> MRVLVTGGSGYIGSHTCVQLLQNGHDVIILDNLCNSKRSVLPVIERLGGKHPTFVEGDIRNEALMTEILHDHAIDTVIHFAGLKAVGESVQKPLEYYDNNVNGTLRLISAMRAANVKNFIFSSAATVYGDQPKIPYVESFPTGTPQSPFGKSKLMVEQILT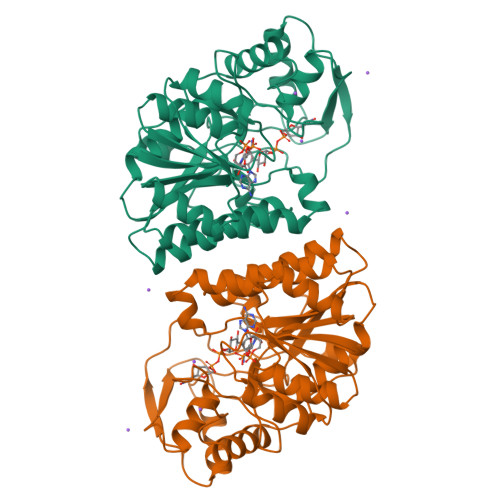DLQKAQPDWSIALLRYFNPVGAHPSGDMGEDPQGIPNNLMPYIAQVAVGRRDSLAIFGNDYPTEDGTGVRDYIHVMDLADGHVVAMEKLANKPGVHIYNLGAGVGNSVLDVVNAFSKACGKPVNYHFAPRREGDLPAYWADASKADRELNWRVTRTLDEMAQDTWHWQSRHPQGYPD> MEQNTTQVFSDLAYKVCFKVINDKNKPFVLHDEQRLA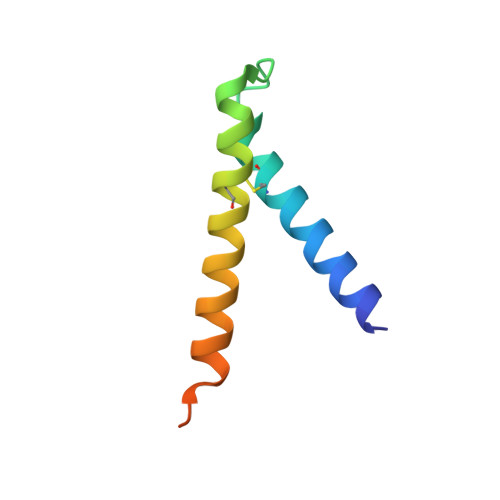NCLTRYVEAFNVTSEYFFRERAGETKVTEKQ>[2x]SLNMFWFLPTHGDGHYLGTEEGSRPVDHGYLQQIAQAADRL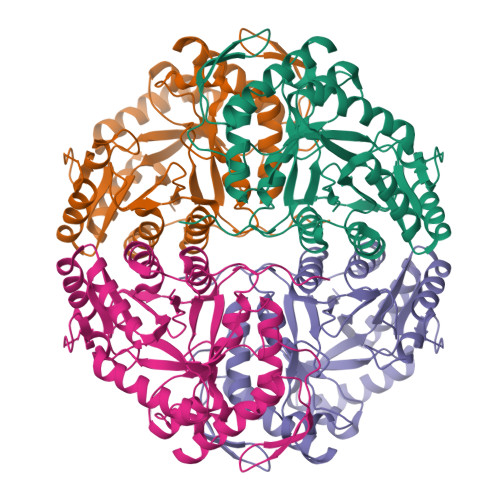GYTGVLIPTGRSCEDAWLVAASMIPVTQRLKFLVALRPSVTSPTVAARQAATLDRLSNGRALFNLVTGSDPQELAGDGVFLDHSERYEASAEFTQVWRRLLQRETVDFNGKHIHVRGAKLLFPAIQQPYPPLYFGGSSDVAQELAAEQVDLYLTWGEPPELVKEKIEQVRAKAAAHGRKIRFGIRLHVIVRETNDEAWQAAERLISHLDDETIAKAQAAFARTDSVGQQRMAALHNGKRDNLEISPNLWAGVGLVRGGAGTALVGDGPTVAARINEYAALGIDSFVLSGYPHLEEAYRVGELLFPLLDVAIPEIPQPQPLNPQGEAVANDFIPRKVAQS3-O-alpha-D-glucopyranosyl-D-fructose | 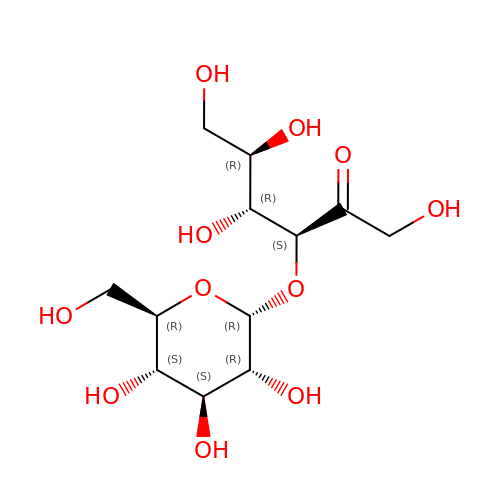C12 H22 O11 | RULSWEULPANCDV-PIXUTMIVSA-N>[4x]AAGVAAWLPFARAAAIGWMPVASGPMPAPPRQERKRTQDALIVLNVSGTRFQTWQDTLERYPDTLLGSSERDFFYHPETQQYFFDRDPDIFRHILNFYRTGKLHYPRHECISAYDEELAFFGLIPEIIGDCCYEEYKDRRRENAERLQDDADTDTAGESALPTMTARQRVWRAFENPHTSTMALVFYYVTGFFIAVSVIANVVETVPCGSSPGHIKELPCGERYAVAFFCLDTACVMIFTVEYLLRLAAAPSRYRFVRSVMSIIDVVAILPYYIGLVMTDNEDVSGAFVTLRVFRVFRIFKFSRHSQGLRILGYTLKSCASELGFLLFSLTMAIIIFATVMFYAEKGSSASKFTSIPAAFWYTIVTMTTLGYGDMVPKTIAGKIFGSICSLSGVLVIALPVPVI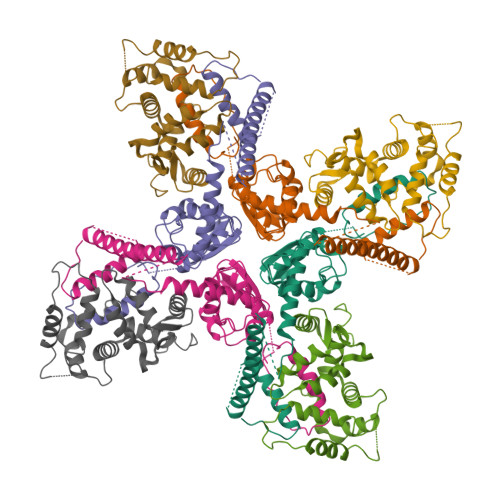VSNFSRIYHQNQRADKRRAQKKARLARIRAAKSGSANAYMQSKRSGLLSNQLQSSEDEQAFVSKSGSSFETQHHHLLHCLEKTTNHEFVD;>[4x]PEGLEQLEAQTNFTKRELQVLYRGFKNECPSGVVNEDTFKQIYAQFFPHGDASTYAHYLFNAFDTTQTGSVKFEDFVTALSILLRGTVHEKLRWTFNLYDINKDGYINKEEMMDIVKAIYDMMGKYTYPVLKEDTPRQHVDVFFQKMDKNKDGIVTLDEFLESCQEDDNIMRSLQLFQNVM>T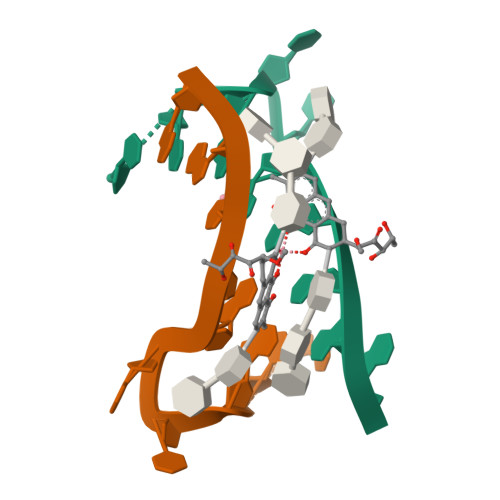CCGCCGCCGA[2x]>[4x]GSLTDLVEQPAKVMRIGTMIKQLLEEVRAAPLDEASRNRLRDIHATSIREL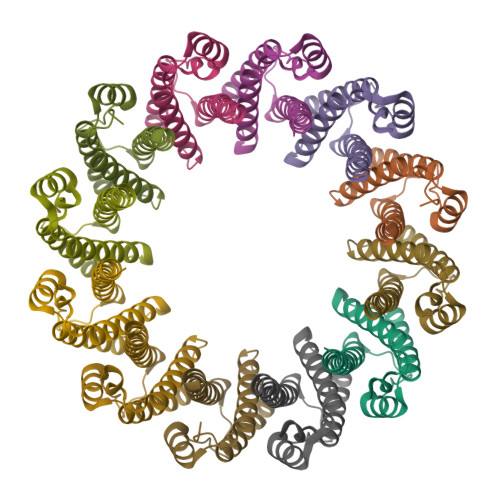EDGLAPELREELDRLTLPFNEDAVPSDAELRIAQAQLVGWLEGLFHGIQTALFAQQMAARAQLQQMRQGALPPG> GSMSPVLTTPKRHAPPPEQLQNVTDFNYTPSHQKPFLQPQAGTTVTTHQDIKQIVEMTLGSEGVLNQAVKLPRGEDENEWLAVHCVDFYNQINMLYGSITEFCSPQTCPRMIATNEYEYLWAFQKGQPPVSVSAPKYVECLMRWCQDQFDDESLFPSKVTGTFPEGFIQRVIQPILRRLFRVYAHIYCHHFNEILELNLQTVLNTSFRHFCLFAQEFELLRPADFGPLLELVMELRDR;> GSASKKLPPKFYERATS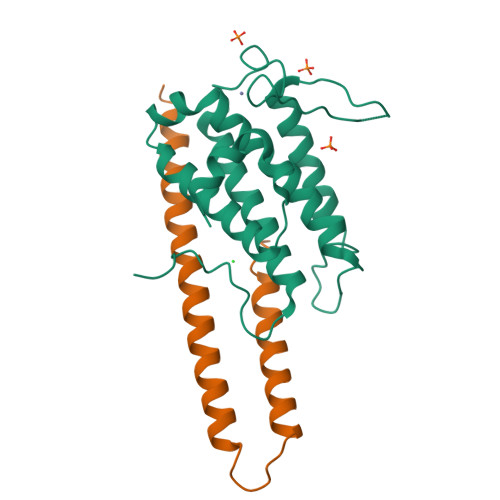NKTQRVVSVCKMYFLEHYCDMFDYVISRRQRTKQVLEYLQQQSQLPNSDQIKLNEEWSSYLQREHQVLRKRRLKPK2-{[(S)-phenylsulfinyl]methyl}benzoic 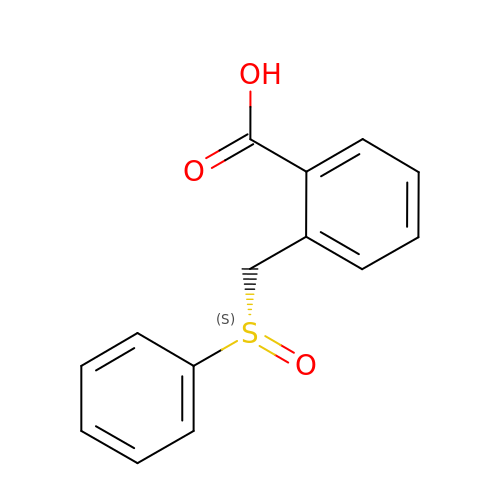acid | C14 H12 O3 S | NNURJXUOUNBQCY-SFHVURJKSA-N> GSQAAHMMSMDFEDFPVESAHRILTPRPTVMVTTVDEEGNINAAPFSFTMPVSIDPPVVAFASAPDHHTARNIESTHEFVINITPADIIERMWVTARDIPAGENELEAAGLAWTSSRRVKPPRIVEAPGHLECELLRMFEVGDHNLITGSVVSASVRSGAVKEGLLDVESVKPVLHVGGNKFVVGDHVRHV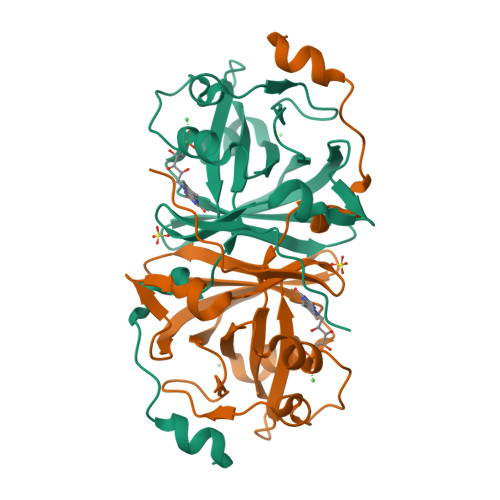E eCGP123 is a bright green FP engineered for extreme stability, and was developed using a two-step process. Phanta was isolated by expression screening of a library targeting amino acid positions 62/63/65/69 and 191/192/193 in the bright green fluorescent protein eCGP123. Phanta contains the substitutions Gln62Met, Thr69Val and His193Gln. The protomers in each protein are typical of the GFP-superfamily and consist of an 11-stranded β-barrel (or β-can) with two small helices forming interconnecting loops protecting the chromophore from bulk solvent.

Collectively, these data indicate that in Phanta the substitution His193Gln plays a key role in reducing ΦF, whilst the substitution Thr69Val is required to suppress formation of the protonated chromophore species observed in eCGP123H193Q. The Phanta chromophore has a pKa of 4 which is significantly lower than that for the other proteins (pKa, 6), and is a desirable property that minimises unwanted pH-driven fluctuations when it is used as a pcFRET acceptor. Omit maps show that the electron density corresponding to the imidazolinone moiety of the chromophore in each of the four protomers of Phanta is well defined. In contrast, there is evidence for disorder around the 4-hyroxybenzyl ring in protomers C and D of the Phanta structure, suggesting that it is mobile within the chromophore cavity. Since a rigid chromophore is considered a prerequisite for efficient fluorescence emission, it is possible the increased mobility observed contributes to the low fluorescence efficiency of Phanta (ΦF, 0.003). Accordingly, in the weakly fluorescent Phanta and eCGP123H193Q the planar network is significantly altered, leaving the chromophore without the underlying scaffold present in eCGP123T69V and eCGP123. In Phanta and eCGP123H193Q, Glu215 no longer interacts with the side chain of Gln193 that replaces the histidine at position 193. Instead a hydrogen bond is formed between the Nδ1 of Gln193 and the Oγ of Ser142, which in turn forms a hydrogen bond with Oη of the chromophore. In Phanta the hydrogen bond network around the chromophore extends from the Oη of the 4-hydroxyphenyl ring to the N2 of the imidazolinone ring, and the O2 of the imidazolinone ring via protein matrix hydrogen bonds involving the side chains of Tyr177, Arg91 and Glu144.

>MSVIKPEMKIKLRMEGAVNGHKFVIEGEGIGKPYEGTQTLDLTVKEGAPLPFSYDILTPAFMYGNRAFVKYPKDIPDYFKQAFPEGYSWERSMTYEDQGICIATSDITMEGDCFFYKIRFDGTNFPPNGPVMQKKTLKWEPSTEKMYVRDGVLKGDVNMALLLEGGGHYRCDFKTTYKAKKDVRLPDAHEVDQRIEILSHDKDYNKVRLYEHAEARYSMLPSQAKASGKPIPNPLLGLDSTHHHHHH[4x]>MMVLVSYDVSTSSPGGDKRLRKVAKACRDLGQRVQFSVFEIEVDPAQWTALRQRLCDLIDPDIDSLRFYHLGAKWEARVEHVGAKPSLDLKGPLIFLEHHHHHH[2x]

Cas2 is a universal Cas protein found in all types of CRISPR-Cas systems, and plays a role in new spacer acquisition during the adaptation stage of CRISPR-Cas immunity. In this study, we describe the structural and functional characterization of Xanthomonas albilineans Cas2 (XaCas2) of a subtype I-C CRISPR-Cas system and provide experimental evidence of pH-dependent conformational switching involving a hinge-bending motion during activation of the dsDNA nuclease function. Overall, the structural features of XaCas2 were similar to those of other subtype I-C Cas2 structures, including the protomer fold, the dimer interface, and the conformational state. The XaCas2 protomer contained an N-terminal ferredoxin fold consisting of a four-stranded antiparallel β-sheet (β1–4) and two α-helices (α1, α2), and a C-terminal segment including a 310-helix (η1) and a β-strand (β5) [Fig. 1(a)]. Although activity was observed under neutral and basic conditions, no dsDNA cleavage was detected at pH 6.0, consistent with the suggestion that the XaCas2 structure crystallized under acidic conditions was in a catalytically inactive conformation. Together, the functional and structural analyses indicate that XaCas2 is a metal- and pH-dependent non-specific dsDNA nuclease, and support the hypothesis that subtype I-C Cas2 proteins undergo a pH-dependent conformational change to allow metal-binding prior to catalysis.

The crystal structures of XaCas2 were determined to resolutions of 1.65 Å and 1.75 Å at 20 and 4 °C, respectively. Data collection and refinement statistics are summarized in Table I. The root mean square deviation (RMSD) of the Cα atomic positions between the two XaCas2 structures was only 0.07 Å, indicating that the two structures were essentially identical. In our crystal structure, XaCas2 seemed to adopt a catalytically inactive conformational state, as was also true of several other subtype I-C Cas2 structures evaluated previously. The crystal structure of the XaCas2 dimer exhibited structural heterogeneity in the putative hinge regions between the two protomers. As the electron densities were well defined and the B factors were relatively low, the two distinct hinge structures of XaCas2 probably represent two stable conformational states, which can be alternatively adopted via movement of the hinge region residues.> MMNAQKSKIALLLAASAVTMALTGCGGSDGNNGNDGSDGGEPAGSIQTLNLDITKVSYENGAPMVTVFATNEADMPVIGLANLEIKKALQLIPEGATGPGNSANWQGLGSSKSYVDNKNGSYTFKFDAFDSNKVFNAQLTQRFNVVSAAGKLADGTTVPVAEMVEDFDGQGNAPQYTKNIVSHEVCASCHVEGEKIYHQATEVETCISCHTQEFADGRGKPHVAFSHLIHNVHNANKAWGKDNKIPTVAQNIVQDNCQVCHVESDMLTEAKNWSRIPTMEVCSSCHVDIDFAAGKGHSQQLDNSNCIACHNSDWTAELHTAKTTATKNLINQYGIETTSTINTETKAATISVQVVDANGTAVDLKTILPKVQRLEIITNVGPNNATLGYSGKDSIFAIKNGALDPKATINDAGKLVYTTTKDLKLGQNGADSDTAFSFVGWSMCSSEGKFVDCADPAFDGVDVTKYTGMKADLAFATLSGKAPSTRHVDSVNMTACANCHTAEFEIHKGKQHAGFVMTEQLSHTQDANGKAIVGLDACVTCHTPDGTYSFANRGALELKLMKKHVEDAYGLIGGNCASCHSDFNLESFKKKGALNTAAAADKTGLYSTPITATCTTCHTVGSQYMVHTKETLESFGAVVDGTKDDATSAAQSETCFYCHTPTVADHTKVKM

For these proteins, a defining feature is close-packed c-type hemes often in van der Waals contact and arranged as approximately linear chains that span the tertiary structure. Shewanella MtrC has evolved to support anaerobic respiration, specifically to deliver electrons from intracellular respiratory chain enzymes to extracellular terminal electron acceptors such as mineral oxides of Fe(III) and Mn(IV) and humic substances. In the native state, MtrC contains 10 optically indistinguishable His/His-ligated hemes.

For this study, we aimed to introduce a spectrally distinct heme within the MtrC heme chain noting that His/Met hemes in their Fe(II) states have a broader, red-shifted Soret band than their His/His-ligated counterparts. Thus, we introduced to MtrC a methionine in place of the distal His561 ligand of Heme 8, Fig. 1A, blue. We were unable to prepare diffracting crystals of Ru-MtrC Met8 or Y657C H561M MtrC. However, diffracting crystals of H561M MtrC could be obtained under similar conditions as for wild-type MtrC, and the structure, resolved to 1.60 Å, confirmed Met561 as the distal ligand of Heme 8 with a Fe-S(Met) distance of 2.3 Å, SI Appendix, Fig. S2. Superposition of the wild-type and mutant protein structures revealed no major global structural differences, with a total main chain rmsd of 0.3 Å as calculated using SUPERPOSE. The rmsd of both main chain and sidechain atoms within 6 Å of hemes 8, 9, and 10 (minus the distal ligand of heme 8) was also calculated, yielding values of 0.2 Å and 0.4 Å, respectively, indicating no significant localized changes surrounding these hemes. A high-potential center (Em +199 ± 16 mV versus standard hydrogen electrode [SHE], error is SEM) was revealed for Ru-MtrC Met8 for which there was no counterpart in Ru-MtrC His8. Introducing a spectrally unique His/Met ligated heme at a site distant from a Ru-photosensitizer has allowed unambiguous detection of intramolecular ET within the MtrC heme chain. Transient absorbance has quantified rate constants for ET between the intervening heme pairs. The values, summarized in Table 3, describe ET between Hemes 10 ↔ 9 and Hemes 9 ↔ 8 with closest edge–edge distances of 3.7 and 4.3 Å, respectively.>[5x]MGNDISLIALLAFSTLLPFIIASGTCFVKFSIVFVMVRNALGLQQIPSNMTLNGVALLLSMFVMWPIMHDAYVYFEDEDVTFNDISSLSKHVDEGLDGYRDYLIKYSDRELVQFFENAQLKRQYGEETETVKRDKDEIEKPSIFALLPAYALSEIKSAFKIGFYLYLPFVVVDLVVSSVLLALGMMMMSPVTISTPIKLVLFVALDGWTLLSKGLILQYMDIAT;> MFYALYFEIHHLVASAALGFARVAPIFFFLPFLNSGVLSGAPRNAIIILVALGVWPHALNEAPPFLSVAMIPLVLQEAAVGVMLGCLLSWPFWVMHALGCIIDNQRGATLSSSIDPANGIDTSEMANFLNMFAAVVYLQNGGLVTMVDVLNKSYQLCDPMNECTPSLPPLLTFINQVAQNALVLASPVVLVLLLSEVFLGLLSRFAPQMNAFAISLTVKSGIAVLIMLLYFSPVLPDNVLRLSFQATGLSSWFYERGATHVLE;>MDDLVFAGNKALYLVLILSGWPTIVATIIGLLVGLFQTVTQLQEQTLPFGIKLLGVCLCLFLLSGWYGEVLLSYGRQVIFLALAKG[4x];>MSIATIVPENAVIGQAVNIRSMETDIVSLDDRLLQAFSGSAIATAVDKQTITNRIEDPNLVTDPKELAISQEMISDYNLYVSMVSTLTRKGVGAVETLLRS[6x];>[17x]MATPWSGYLDDVSAKFDTGVDNLQTQVTEALDKLAAKPSDPALLAAYQSKLSEYNLYRNAQSNTVKVFKDIDAAIIQNFR

Many important human pathogens including Salmonella, Shigella, Yersinia, and enteropathogenic Escherichia coli employ a conserved, virulent type III secretion system (T3SS), also commonly referred to as the injectisome, to deliver a pleiotropic arsenal of proteins into target eukaryotic cells. Chaperones present effector proteins in a non-globular, secretion-competent state to a cytoplasmic sorting platform complex, which sorts and loads effectors into the export apparatus (EA) subcomplex located inside the membrane-bound basal body. The basal body and the needle filament, collectively termed the needle complex, function as a continuous conduit for effector protein translocation from the prokaryotic to the host cell cytoplasm. Besides its role as a translocon, the EA also functions as a structural scaffold onto which the inner rod protein PrgJ assembles.

In the apo-state, a unique loop of residues 106-123 of SpaR extends horizontally out on top of the M-gate. Consistent with the recombinant EA from Shigella flexneri injectisomes, SpaR residues Leu110 and Ile114 (Phe110 and Phe113 in FliP) interface with the methionines of the M-gate below, creating what has been termed a plug in the structurally-related flagellar system. Intriguingly, our apo- and translocation-state EAs superimpose with a low root mean square deviation (rmsd) of 0.49 Å (SpaP : Q : R), revealing that in fact only subtle conformational changes are needed to facilitate substrate transport through the channel of the needle complex. In fact, many residues involved in substrate translocation localize to loop regions, which together with low rmsd values between apo-state and substrate-engaged structures supports the concept that the basal body rings and the bulk of the SpaPQR complex provide a scaffold to position critical residues in the secretion channel. Our data confirms the M-gate forms the main constriction in apo-state structures that shifts just enough to allow substrate passage while likely preventing unwanted transport of other molecules. (3) The SpaR loop, resting above the M-gate and blocking the channel, extends upwards, assuming an open conformation, which together with the surrounding Q2-belt creates an interface to engage the substrate. Six PrgJ protomers interface with 1 + 5 SpaR and  P proteins and previously unresolved lipids, together creating the atrium. The lipids reside in a circular gap present in the upper EA, where they function to accommodate SpaP α-helix α1 and stabilize the helical fork of PrgJ, together forming a nucleation seed that drives polymerization of the needle filament. Notably, the lowest monomer PrgJ1 has a unique fold, which extends horizontally, interfacing the SpaR loop connecting α-helices α2 and α3 before traversing SpaP1 to then cross the gap between the EA and the basal body, clarifying earlier reports in which this part could not be resolved and PrgJ2 was speculated to interface in alternate locations.> MSEDKAKLGTTRSATEYRLS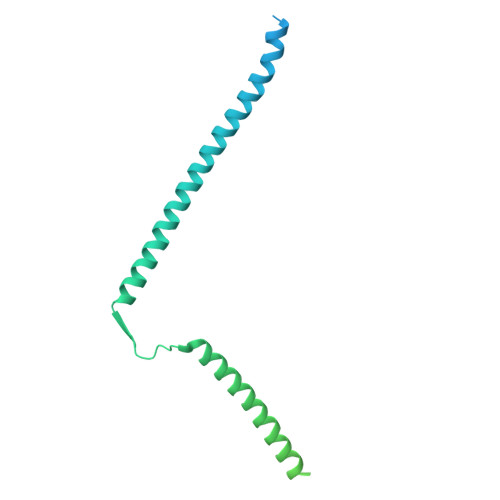IGSAPTSRRSSMGESSSLMKFADQEGLTSSVGEYNENTIQQLLLPKIRELSDSIITLDSNFTRLNFIHESLADLNESLGSLLYGIMSNSWCVEFSQAPHDIQDDLIAIKQLKSLEDEKNNLVMELSNMERGIKRKKDEQGENDLAKASQNKQFNQPLFPSSQVRKYRSYDNRDKRKPSKIGNNLQVENEEDYEDDTSSEASFVLNPTNIGMSKSSQGHVTKTTRLNNNTNSKLRRKSILHTIRNSIASGADLPIENDNVVNLGDLHPNNRISLGSGAARVVNGPVTKNRNSMFSGRAERKPTESRHSVAKKTEKKINTRPPFR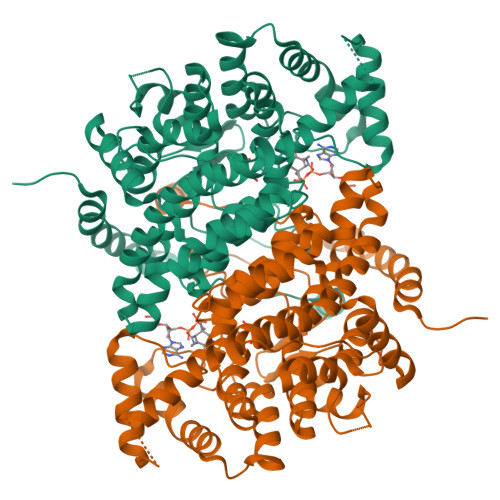> ASSTNLKDVLAALIPKEQARIKTFRQQHGGTALGQITVDMSYGGMRGMKGLVYETSVLDPDEGIRFRGFSIPECQKLLPKGGXGGEPLPEGLFWLLVTGQIPTGAQVSWLSKEWAKRAALPSHVVTMLDNFPTNLHPMSQLSAAITALNSESNFARAYAEGILRTKYWEMVYESAMDLIAKLPCVAAKIYRNLYRAGSSIGAIDSKLDWSHNFTNMLGYTDAQFTELMRLYLTIHSDHEGGNVSAHTSHLVGSALSDPYLSFAAAMNGLAGPLHGLANQEVLGWLAQLQKAXXXAGADASLRDYIWNTLNSGRVVPGYGHAVLRKTDPRYTCQREFALKHLPGDPMFKLVAQLYKIVPNVLLEQGAAANPWPNVDAHSGVLLQYYGMTEMNYYTVLFGVSRALGVLAQLIWSRALGFPLERPKSMSTDGLIAL> FSPQLLSLLSLKTSLSGPPSAFQDWKVPVNGQNDAVWCSWSGVVCDNVTAQVISLDLSHRNLSGRIPIQIRYLSSLLYLNLSGNSLEGSFPTSIFDLTKLTTLDISRNSFDSSFPPGISKLKFLKVFNAFSNNFEGLLPSDVSRLRFLEELNFGGSYFEGEIPAAYGG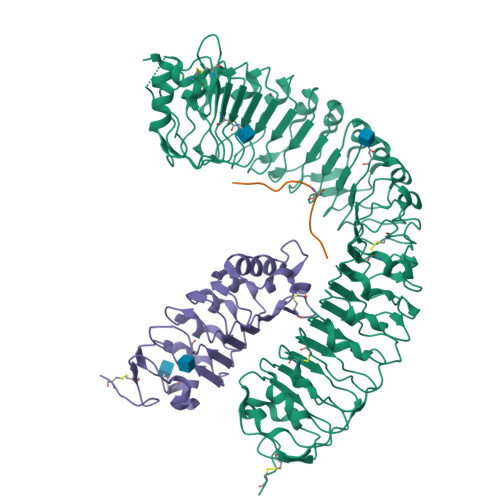LQRLKFIHLAGNVLGGKLPPRLGLLTELQHMEIGYNHFNGNIPSEFALLSNLKYFDVSNCSLSGSLPQELGNLSNLETLFLFQNGFTGEIPESYSNLKSLKLLDFSSNQLSGSIPSGFSTLKNLTWLSLISNNLSGEVPEGIGELPELTTLFLWNNNFTGVLPHKLGSNGKLETMDVSNNSFTGTIPSSLCHGNKLYKLILFSNMFEGELPKSLTRCESLWRFRSQNNRLNGTIPIGFGSLRNLTFVDLSNNRFTDQIPADFATAPVLQYLNLSTNFFHRKLPENIWKAPNLQIFSASFSNLIGEIPNYVGCKSFYRIELQGNSLNGTIPWDIGHCEKLLCLNLSQNHLNGIIPWEISTLPSIADVDLSHNLLTGTIPSDFGSSKTITTFNVSYNQLIGPIPSGSFAHLNPSFFSSNEGLCGDLVGKPCN;> HEVPSGPNPISN;> NMEGDALHSLRANLVDPNNVLQSWDPTLVNPCTWFHVTCNNENSVIRVDLGNADLSGQLVPQLGQLKNLQYLELYSNNITGPVPSDLGNLTNLVSLDLYLNSFTGPIPDSLGKLFKLRFLRLNNNSLTGPIPMSLTNIMTLQVLDLSNNRLSGSVPDNGSFSLFTPISFANNLDLCGPVTSRPCP>[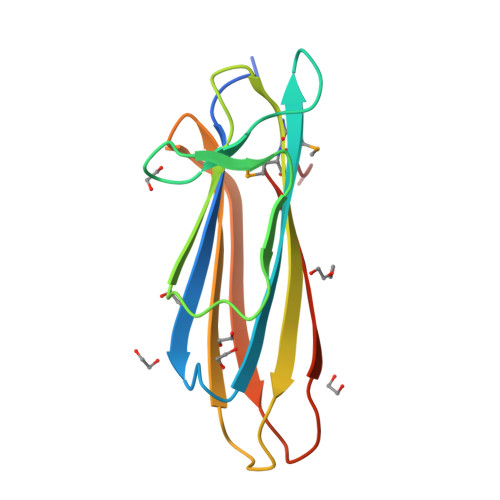10x]GNDDDNKNTTGVHKIVVEQSGNTDDFDLNIAFGAANTGGVAKLYNENGEYLGDSYLVNKVTENKISCQTGKEGSMMTCAGSVISTSEQAGKKLKISVIAYIDNKEVNRLEKEYITKGSTLVENFSVSTTSVE> GHHHHHHHHHHSSGHISGDAMEDKQERANYEKLQQKFQMLMSKHQAHVRPQFESLEKINKDIVGWIKLSGTSLNYPVLQGKTN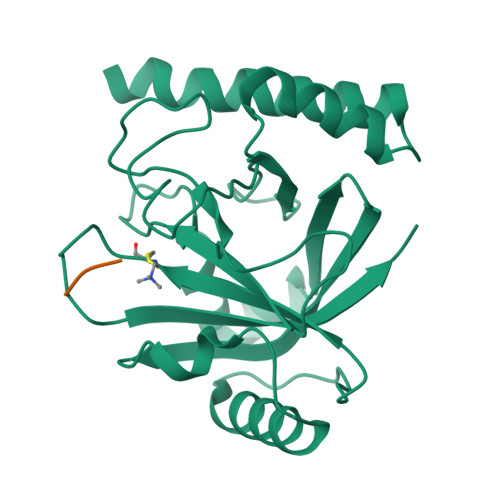HDYLNLDFEREHRRKGSIFMDFRNELKNLNHNTILYGHHVGDNTMFDVLEDYLKQSFYEKHKIIEFDNKYGKYQLQVFSAYKTTTKDNYIRTDFENDQDYQQFLDETKRKSVINSDVNVTVKDRIMTLSTCEDAYSETTKRIVVVAKIIKVS;> GGG>MSKIESALQAAQPGLSRLRGGAGGMGYRAATTQAEQPRSSLLDTIGRFAKAGADMYTAKEQRARDLADERSNEIIRKLTPEQRREALNNGTLLYQDDPYAMEALRVKTGRNAAYLVDDDVMQKIKEGVFRTREEMEEYRHSRLQEGAKVYAEQFGIDPEDVDYQRGFNGDITERNISLYGAHDNFLSQQAQKGAIMNSRVELNGVLQDPDMLRRPDSADFFEKYIDNGLVTGAIPSDAQATQLISQAFSDASSRAGGADFLMRVGDKKVTLNGATTTYRELIGEEQWNALMVTAQRSQFETDAKLNEQYRLKINSALNQEDPRTA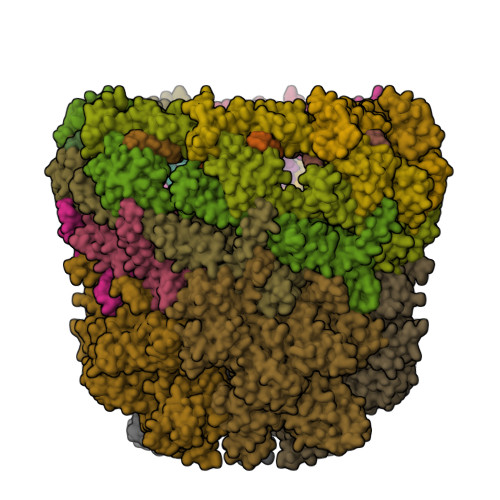WEMLQGIKAELDKVQPDEQMTPQREWLISAQEQVQNQMNAWTKAQAKALDDSMKSMNKLDVIDKQFQKRINGEWVSTDFKDMPVNENTGEFKHSDMVNYANKKLAEIDSMDIPDGAKDAMKLKYLQADSKDGAFRTAIGTMVTDAGQEWSAAVINGKLPERTPAMDALRRIRNADPQLIAALYPDQAELFLTMDMMDKQGIDPQVILDADRLTVKRSKEQRFEDDKAFESALNASKAPEIARMPASLRESARKIYDSVKYRSGNESMAMEQMTKFLKESTYTFTGDDVDGDTVGVIPKNMMQVNSDPKSWEQGRDILEEARKGIIASNPWITNKQLTMYSQGDSIYLMDTTGQVRVRYDKELLSKVWSENQKKLEEKAREKALADVNKRAPIVAATKAREAAAKRVREKRKQTPKFIYGRKE[8x];>[4x]MDKYDKNVPSDYDGLFQKAADANGVSYDLLRKVAWTESRFVPTAKSKTGPLGMMQFTKATAKALGLRVTDGPDDDRLNPELAINAAAKQLAGLVGKFDGDELKAALAYNQGEGRLGNPQLEAYSKGDFASISEEGRNYMRNLLDVAKSPMAGQLETFGGITPKGKGIPAEVGLAGIGHKQKVTQELPESTSFDVKGIEQEATAKPFAKDFWETHGETLDEYNSRSTFFGFKNAAEAELSNSVAGMAFRAGRLDNGFDVFKDTITPTRWNSHIWTPEELEKIRTEVKNPAYINVVTGGSPENLDDLIKLANENFENDSRAAEAGLGAKLSAGIIGAGVDPLSYVPMVGVTGKGFKLINKALVVGAESAALNVASEGLRTSVAGGDADYAGAALGGFVFGAGMSAISDAVAAGLKRSKPEAEFDNEFIGPMMRLEARETARNANSADLSRMNTENMKFEGEHNGVPYEDLPTERGAVVLHDGSVLSASNPINPKTLKEFSEVDPEKAARGIKLAGFTEIGLKTLGSDDADIRRVAIDLVRSPTGMQSGASGKFGATASDIHERLHGTDQRTYNDLYKAMSDAMKDPEFSTGGAKMSREETRYTIYRRAALAIERPELQKALTPSERIVMDIIKRHFDTKRELMENPAIFGNTKAVSIFPESRHKGTYVPHVYDRHAKALMIQRYGAEGLQEGIARSWMNSYVSRPEVKARVDEMLKELHGVKEVTPEMVEKYAMDKAYGISHSDQFTNSSIIEENIEGLVGIENNSFLEARNLFDSDLSITMPDGQQFSVNDLRDFDMFRIMPAYDRRVNGDIAIMGSTGKTTKELKDEILALKAKAEGDGKKTGEVHALMDTVKILTGRARRNQDTVWETSLRAINDLGFFAKNAYMGAQNITEIAGMIVTGNVRALGHGIPILRDTLYKSKPVSAKELKELHASLFGKEVDQLIRPKRADIVQRLREATDTGPAVANIVGTLKYSTQELAARSPWTKLLNGTTNYLLDAARQGMLGDVISATLTGKTTRWEKEGFLRGASVTPEQMAGIKSLIKEHMVRGEDGKFTVKDKQAFSMDPRAMDLWRLADKVADEAMLRPHKVSLQDSHAFGALGKMVMQFKSFTIKSLNSKFLRTFYDGYKNNRAIDAALSIITSMGLAGGFYAMAAHVKAYALPKEKRKEYLERALDPTMIAHAALSRSSQLGAPLAMVDLVGGVLGFESSKMARSTILPKDTVKERDPNKPYTSREVMGAMGSNLLEQMPSAGFVANVGATLMNAAGVVNSPNKATEQDFMTGLMNSTKELVPNDPLTQQLVLKIYEANGVNLRERRK;>[8x]MCWAAAIPIAISGAQAISGQNAQAKMIAAQTAAGRRQAMEIMRQTNIQNADLSLQARSKLEEASAELTSQNMQKVQAIGSIRAAIGESMLEGSSMDRIKRVTEGQFIREANMVTENYRRDYQAIFAQQLGGTQSAASQIDEIYKSEQKQKSKLQMVLDPLAIMGSSAASAYASGAFDSKSTTKAPIVAAKGTKTGR> SVRPWEFRKVIQAEYRERLPRNYELKHWKKPSKIMIGSILRLLETNTVSALDSVFEKYEKEMNQMTHGDN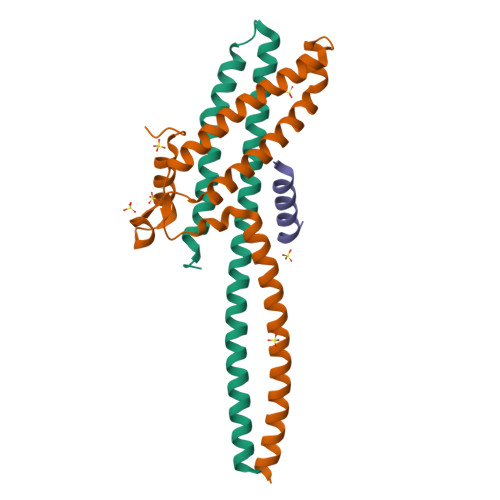NEVKRIYSKKERLLEIILTKIKKKLRQAKFPSRISERDLDIEYIYSKRQFIQNRYSQELQNNERLEAILSREQNLLEETRKL;> LSSSITSVTTIDVLSSLFINLFENDLIPQALKDFNKSDDDQFRKLLYKLDLRLFQTISDQMTRDLKDILDINVSNNELCYQLKQVLARKEDLNQQIISVRNEIQELK;> QSINDRALSLLQRTRATK>MNHKHHHHHHSSGENLYFQGHMSKVKLTKENIVALLTQGKDLEFEENQNLVAFNFKTFCLENLDQIKKMSIISCLTFLKNRQSIMKVIKQSDFTFGKITIKKTSDRIGATDMTFRRLDSLIRVRLVEETGNSENLNTIKSKIASHPLIQAYGLPLDDAKSVRLAIMLGGSLPLIASVDSFEMISVVLAIYQDAKYKDLGIDPKKYDTKEALGKVCTVLKSKAFEMNEDQVKKGKEYAAILSSSNPNAKGSVAMEHYSETLNKFYEMFGVKKQAK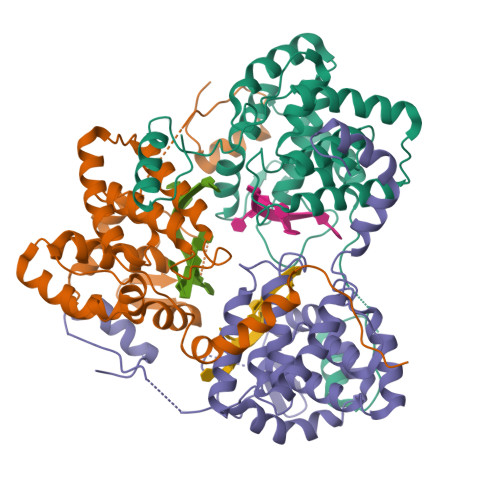LAELA[3x]> EIASEYLGGPGGDAFDDKAVAQNGDITRIEMQCTDVATYIKLRYGKVDSRQWGWGNENCIQWSKKGEKVVHELSSGEYITSAIVTYGKYVQSITFKTNKRTLPRCGTSATEKSVTVLIPGGLKYISGRWGCRIDGLRFHAKC;> QVASEYLGGPGGDAFDDKALAQNGDITRIEMQCTDVATYIKLRYGKVDSRQWGWANENCIQWSKKGVKVVHELSSGEYITSAIVTYGKYVQSITFKTNKRTLPRCGTSATEKSVTVLIPGGLKYISGRWGCRIDGL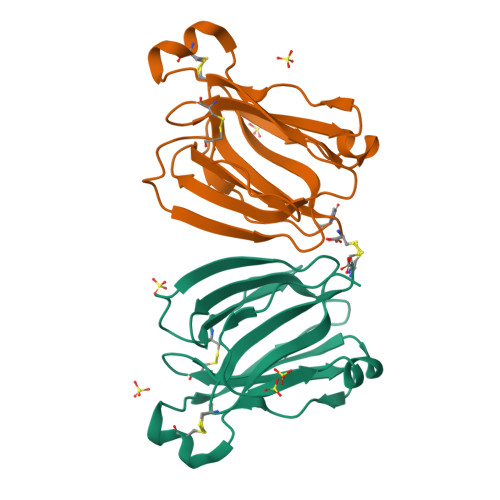RFHAKC> GSPSRAEYRNWSKPQCDITGFAPFSKDNSIRLSAGGDIWVTREPYVSCDPDKCYQFALGQGTTLNNVHSNNTVRDRTPYRTLLMNELGVPFHLGTKQVCIAWSSSSCHDGKAWLHVCITGDDKNATASFIYNGRLVDSVVSWSKEILRTQESECVCINGTCTVVMTDGSASGKADTKILFIEEGKIVHTSTLSGSAQHVEECSCYPRYPGVRCVCRDNWKGSNRPIVDINIKDHSIVSSYVCSGLVGDTPRKNDSSSSSHCLD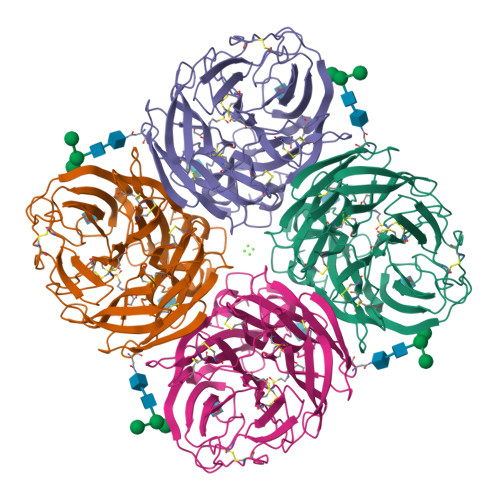PNNEEGGHGVKGWAFDDGNDVWMGRTINETSRLGYETFKVIEGWSNPKSKLQINRQVIVDRGNRSGYSGIFSVEGKSCINRCFYVELIRGRKEETEVLWTSNSIVVFCGTSGTYGTGSWPDGADLNLMPI> WESKFSKEGLTFDDVLLVPAKSEVLPRDVDLSVELTKTLKLNIPVISAGMDTVTESAMAIAMARQGGLGIIHKNMSIEQQAEQVDKVKRSERGITNPFFLTPDHQVFDAEHLMGKRISGVPIEEDLVGIITNRDLRFISMKISDVMTKEELVTASVGTTLDEAEKILQKHKIEKLPLVGLITIKDIEKVIEFPNSSKDIHGRLIVGAAVGVTGDTMTRVKKLVEANVDVIVIDTAHGHSQGVLNTVTKIRETYPELNIIAGNVATAEATRALIEAGADVVKVGIGPICTTRVVAGVGVPQITAIYDCATEARKHGKTIIADGGIKFSGDITKALAAGGHAVMLGSLLAGT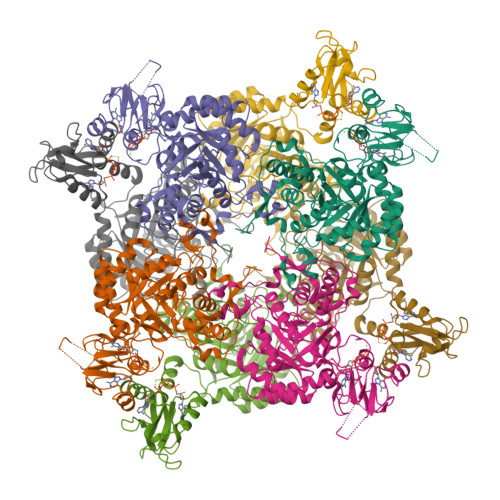SESPGETPYKGPVEETVYQLVGGLRSGMGYCGSKDLRALREEAQFIRMTGA;> HHWESKFSKEGLTFDDVLLVPAKSEVLPRDVDLSVELTKTLKLNIPVISAGMDTVTESAMAIAMARQGGLGIIHKNMSIEQQAEQVDKVKRSERGITNPFFLTPDHQVFDAEHLMGKYRISGVPIVNNEEDQKLVGIITNRDLRFIADYSMKISDVMTKEELVTASVGTTLDEAEKILQKHKIEKLPLVDDQNKLKGLITIKDIEKVIEFPNSSKDIHGRLIVGAAVGVTGDTMTRVKKLVEANVDVIVIDTAHGHSQGVLNTVTKIRETYPELNIIAGNVATAEATRALIEAGADVVKVGIGPGSICTTRVVAGVGVPQITAIYDCATEARKHGKTIIADGGIKFSGDITKALAAGGHAVMLGSLLAGTSESPGAAAAPYKGPVEETVYQLVGGLRSGMGYCGSKDLRALREEAQFIRMTGAAA>[2x]MGHHHHHHEFNIR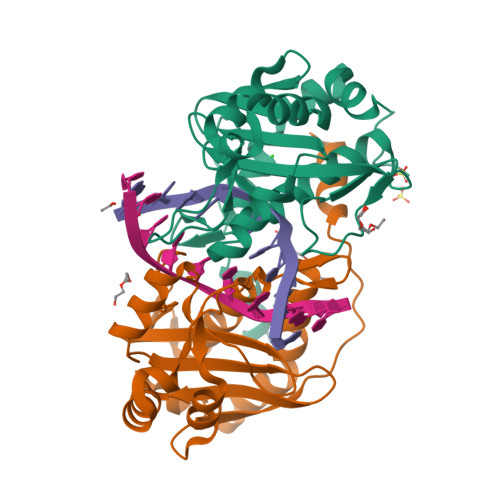DRMNDHLKDLFRDRLIIDKVQRRLPYMFQLAELESSRAGKVGMEVGSLRERIISSLLIYKFGEKNVETDLPITEPEIDVKLFGSPISIKTITGKEPAGVKLIWTVDATKARQFLETWHPRFDLILVHINWSSLGGVYYIPDYVQQRIFDEIGKDKYIKLPKQGTNPRGVEISNEALKEIMTDEETMSIKIEWKKTNVQYNAFKRWVDLWSEG> DHQLL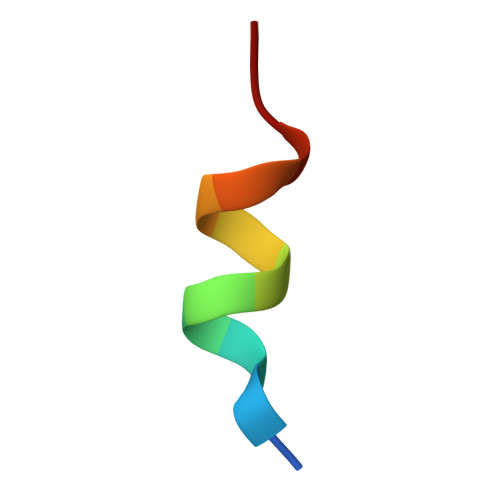RYLLDKD({[(chloromethyl)sulfonyl]amino}methyl)boronic acid | C2 H7 B Cl N O4 S | 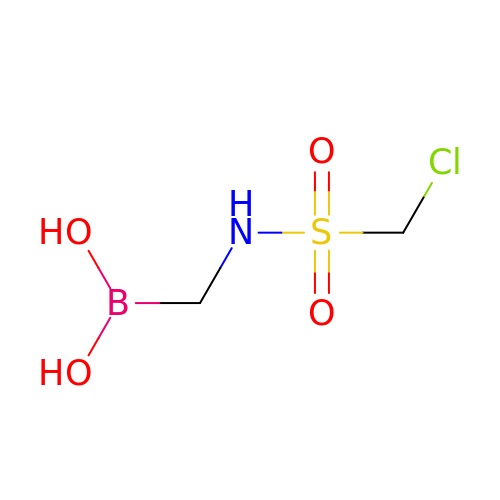DYDOICABPAYWAK-UHFFFAOYSA-N>[2x]MKKFIFSLLATLISFSVFAQSADDTYVVNKADGTSQSYKVMEFPNIKFNGDGTFGNYMTGFDDFGQINVWNISDVKSVTFNIAHSNPVDVSGVFLADASANDAAKKLYKYLRLVYGNKILSGMMAHVAWNHDEADKIHVLTGKYPAINCYDFIHIAVPNQGSNGWINYNDITPVTEWADAGGIVSLMWHFNVPQNENTTIGADGSGQGINSSQTTFKASHALVSGTWENKFFMEQMENVANVILKLQDAGIVALWRPFHEAAGNATLKSGANWGKAWFWWGEDGPDVYKQLWHTMFNYFSNKGIHNLIWEWTSQNYNGDSDIYNNDDDWYPGDAYVDIIGRDLYGTTAVQQYSEYSQLKGRYPSKMIALAECGVNN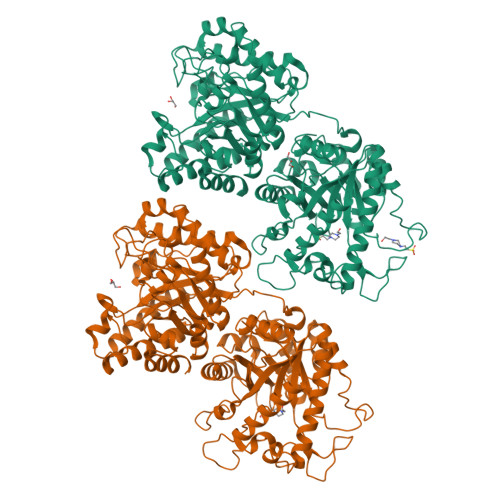STITADVEQAWNAGAKWLNFMPWYGESMPSDEWWTKVMNENVVITRDEINQNATYMEESAQSAVDNFGLGFNLGNTLDANGCGTGKPVATYETFWGQPETTQDMMTFLMQNGFNAVRIPVTWYEHMDAEGNVDEAWMMRVKAIVEYAMNAGLYAIVNVHHDTAAGSGAWIKADTDVYAATKEKFKKLWTQIANALADYDQHLLFEGYNEMLDGNNSWDEPQKASGYEALNNYAQDFVDAVRATGGNNATRNLIVNTYAAAKGENVLNNFMLPTDAVNNHLIVQVHSYDPWNFFNTKTTWDSECHNTLTEIFSALSKKFTTIPYIIGEYGTHGESDISVSKSSPAEKIKLAADQAADMVKLAKDHHSATFYWMSIFDGSDRIQPQWSLPTVVEAMQEAYNN The structural studies herein confirmed SAV0551 from S. aureus Mu50 as a member of the DJ-1 superfamily and that it has all the pertinent traits of this group, including the sandwich fold and nucleophilic arm. It specifically belongs to the Hsp-type subfamily because of the presence of cap domain and aspects of its dimeric interface. The results demonstrate that SAV0551 is a glyoxalase III that produces non-toxic D-lactate from toxic methylglyoxal independent of any cofactors. SAV0551 shows chaperone activity regardless of active site mutations, whereas the catalytic cysteine and active site residues are crucial for its glyoxalase III function.

The crystal structure of SAV0551 was determined at 2.6 Å resolution including the additional C-terminal histidine tag. The asymmetric unit contains eight molecules and each of them consists of two domains: a core domain whose similarity to DJ-1 superfamily proteins had been expected and a cap domain, which is also called the ‘P’ region. The core domain consists of an α/β sandwich fold with nine α-helices and six β-strands. Additionally, four short α-helices (α1 (residues 26–32), α3 (residues 110–112), α10 (residues 218–222), and α11 (residues 224–227)) and two β-strands (β2 (residues 64–66) and β3 (residues 72–74)) form the cap domain. The core and cap domains are linked via a 22-residue long-linker (residues 33–53). Cys190 and His191 from the core domain and Asp221 from cap domain constitute a catalytic triad. The Cys190 Sγ interacts with the His191 Nδ1, while the Asp221 carboxylate hydrogen bonds with His191 Nε2. The crystal structure shows that SAV0551 is a compact homodimer. The loops (residues 1–25 and 67–71) and β-strands (β2 (residues 64–66) and β3 (residues 72–74)) from cap domain are responsible for dimer formation. SAV0551 has a deep acidic canyon that winds from the dimeric interface to each side of the subunit, and bowl structure is located on the bottom side.

>MSQDVNELSKQPTPDKAEDNAFFPSPYSLSQYTAPKTDFDGVEHKGAYKDGKWKVLMIAAEERYVLLENGKMFSTGNHPVEMLLPLHHLMEAGFDVDVATLSGYPVKLELWAMPTEDEAVISTYNKLKEKLKQPKKLADVIKNELGPDSDYLSVFIPGGHAAVVGISESEDVQQTLDWALDNDRFIVTLCHGPAALLSAGLNREKSPLEGYSVCVFPDSLDEGANIEIGYLPGRLKWLVADLLTKQGLKVVNDDMTGRTLKDRKLLTGDSPLASNELGKLAVNEMLNAIQNKLEHHHHHH[8x]Noroviruses are highly contagious, infecting both humans and animals. The human norovirus capsid protruding (P) domain binds histo-blood group antigen (HBGA) co-factors for infection, and a recently discovered bat norovirus (GX) was also found to interact with HBGAs. In this study, we determined the P domain structures of four human noroviruses and one bat norovirus using X-ray crystallography to examine structural features linked to potential interspecies transmission. The principal structural difference was a variable length P2 subdomain loop (Loop A), which was located near the HBGA pocket.

The P domains of GII.9 (AY038599), GII.23 (KT290889), GII.27 (MG495077), GVIII (AJ844470), and GX (MF373609) were expressed in E.coli. The five P domains were structurally equivalent with a root mean square deviation for C-alpha atoms ranging between 0.586 Å (GII.23-GII.27) and 1.645 Å (GII.9-GX). The cross-reactivity of the P domains was determined using direct ELISA with a broad-spectrum human norovirus Nanobody (Fc-NB26) that binds to a highly conserved region on the P domain. Fc-NB26 bound to GII.9, GII.23, and GII. P domains in a dose-dependent manner at concentrations less than 80 ng/mL. Structural modeling of the Fc-NB26-binding site indicated that GII.9, GII.23, and GII. P domains contained most of the equivalent residues that could interact with Fc-NB26. Our cumulative data show that Fc-NB26/NB26 binds most GII genotypes, and the epitope is vulnerable and a therapeutic target region for GII noroviruses.

>[2x]KAFTIPVLKISEMTNSRFPVPVDQMYTSRSEGIVVQPQNGRATIDGELLGTTLVSPVSVCNFKGNLQAEVPGQHQLYQLQLTNLDGSPIDPTDDTPGPLGCPDFTGLLYGVASQRGPGDATRAHEARIDTGSDTFAPKIGQVRFYSTSSDFETNQPTHFTPIGIYIEGNSSDFNQWQLPRYGGHLANNNHLAPAVSPLFPGEQILFFRSFIPGASGHTNGEMDCLLPQEFVQHFYQEAATARSEVALLRFVNPDTGRALFESKLHKQGFMTIASSGDHPIIMPTNGYFRFEAWVNQFYSLAPV> MLSKVTRRFLNYNQIYCFASQHGAEHHKLTASDEAYLNEVRQRYVTPDMEKWAYLDYKKHPSTTLSHYDHKSKDYVESERDDYNADVATNSHNKLIDDFKRNLQMQRKVHDILQKMDRPYLRGVPGVTKNISAGLQDYSAPVSKKSQSDPNDFYRDAYRNENRWIDQSVFTPKTSKMTHYDVEWPKELASRPVTKKFHHDKGYKYDVTT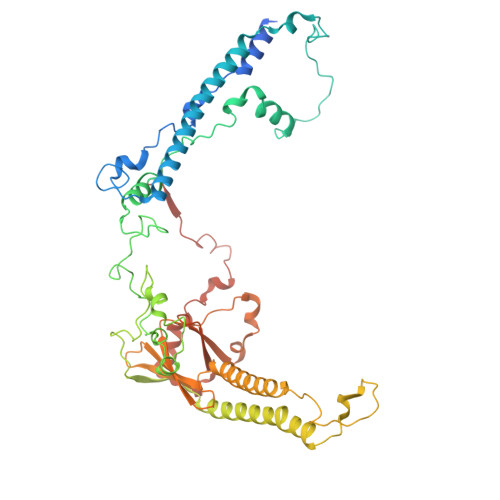PYDQRYNYVADRLGHPEILGNPFERLMRLEGDIYHPNYLDQPFVKVPNANPNASLNFEEGEVLYENTRLLEWAKFWNYSVVVGYLWCAYFVPYNIFFKTHMPLEHAYDNLFFPYFQHTHFLWDNNALHIPTVGGVAIYATYIALSYINNIWKDYVVRAQFSKDKELLFVTRVSPFGTTEEEVYEVAHLEHLPPSVRSGVKDLSAQDADGLVDVTCMSSQRSLVFYKGDQYWNPKVYNDFINQTSNLWTRNYTGYNRLEVQNSVEQVKIGFSHSSQPKLEKK> 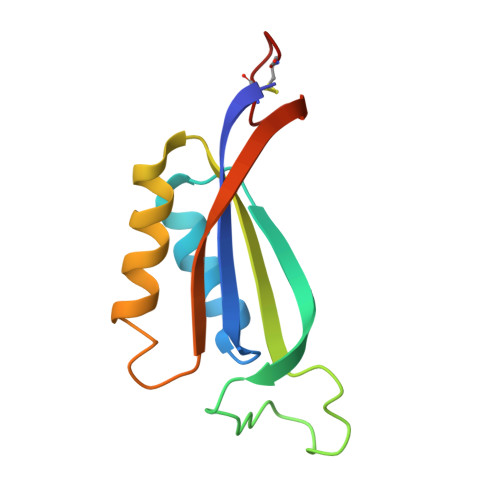MAKPANKLVIVTEKILLKKIAKIIDESGAKGYTVMNTGGKGSRNVRSSGQPNTSDIEANIKFEILTETREMAEEIADRVAVKYFNDYAGIIYICSAEVLYGHTFCGPEGC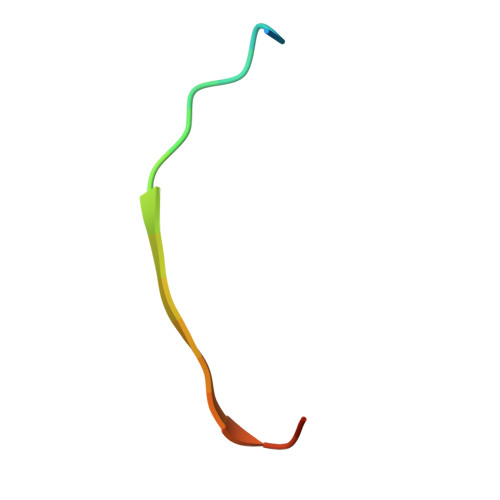> DEQSGISQTVIVGPWGAKSS> MFGLIGHLTSLEQARDVSRRMGYDEYADQGLEFWSSAPPQIV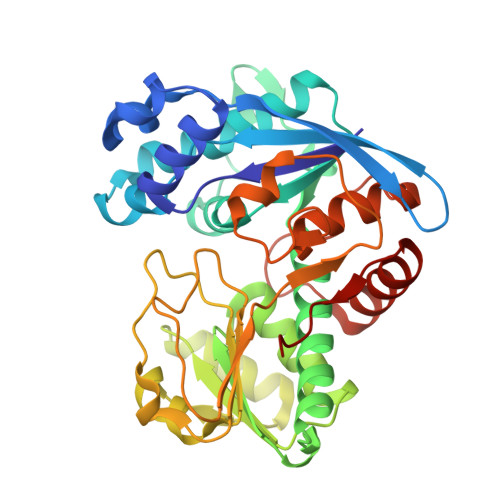DEITVTSATGKVIHGRYIESCFLPEMLAARRFKTATRKVLNAMSHAQKHGIDISALGGFTSIIFENFDLASLRQVRDTTLEFERFTTGNTHTAYVICRQVEAAAKTLGIDITQATVAVVGATGDIGSAVCRWLDLKLGVGDLILTARNQERLDNLQAELGRGKILPLEAALPEADFIVWVASMPQGVVIDPATLKQPCVLIDGGYPKNLGSKVQGEGIYVLNGGVVEHCFDIDWQIMSAAEMARPERQMFASFAEAMLLEFEGWHTNFSWGRNQITIEKMEAIGEASVRHGFQPLALAI> IVGGYTCEENSLPYQVSLNSGSHFCGGSLISEQWVVSAAHCYKTRIQVRLGEHNIKVLEGNEQFINAAKIIRHPKYNRDTLDNDIMLIKLSSPAVINARVSTISLPTAPPAA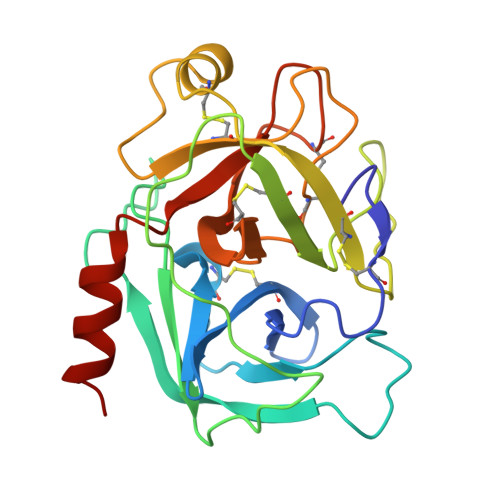GTECLISGWGNTLSFGADYPDELKCLDAPVLTQAECKASYPGKITNSMFCVGFLEGGKDSCQRDAGGPVVCNGQLQGVVSWGHGCAWKNRPGVYTKVYNYVDWIKDTIAANS> AKVVKFSYMWTINNFSFCREEMGEVIKSSTFSSGANDKLKWCLRVNPKGLDEESKDYLSLYLLLVSCPKSEVRAKF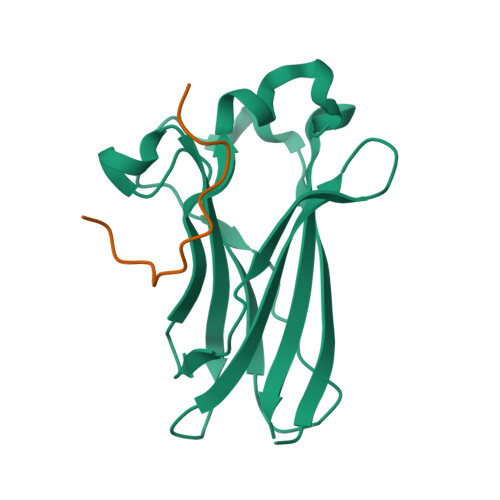KFSILNAKGEETKAMESQRAYRFVQGKDWGFKKFIRRDFLLDEANGLLPDDKLTLFCEVSVVQD;> AEKPLQVAAVDSSVPRT> MSQISKTHSRLAGRNAKPFDLKNITNDAVASLSRIGLVFDHAVVQDQIKALAKAGAFRSGSAMDSNFTAPVTTPSIPTPIQFLQTWLPGFVKVMTAARKIDEIIGIDTVGSWEDQEIVQGIVEPAGTAVEYGDHTNIPLTSWNANFERRTIVRGELGMMVGTLEEGRASAIRLNSAETKRQQAAIGLEIFRNAIGFYGWQSGLGNRTYGFLNDPNLPAFQTPPSQGWSTADWAGIIGDIREAVRQLRIQSQDQIDPKAEKITLALATSKVDYLSVTTPYGISVSDWIEQTYPKMRIVSAPELSGVQMKAQEPEDALVLF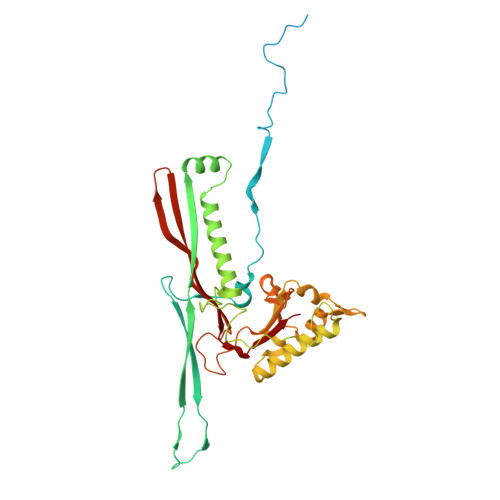VEDVNAAVDGSTDGGSVFSQLVQSKFITLGVEKRAKSYVEDFSNGTAGALCKRPWAVVRYLGI4-{4-[4-(3,4-difluorophenyl)piperidine-1-sulfonyl]phenyl}-4-oxobutanoic 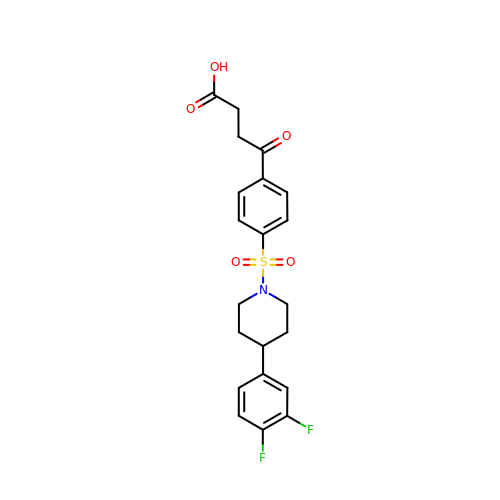acid | C21 H21 F2 N O5 S | MCLQTWVCUVNNQM-UHFFFAOYSA-N> MAQQDGPTPEPSVGSRTVLVYMIAQNSLAPLASADIEEMKEGMRQVDATSGNLLVYIDDYSAPRLIRLGKDKKGKVVEETIENYPEQNSADANVMKKVISTAFNQYKAEKYGMVFWSHGEGWIPSPAKTR;> WFGQDGNNYMDIADLHAALQVAPDLDFLFFDACFMEAVEVAYALRDCGSYLISSPTEIPGPGAPYQTVVPAMFSAENAALKIASCYYDYYQSRYDDGIGMSNEDWTGGVSVGVAKMSELENLAVATSKVLPRYITGKQNFDLSGVMCYDRRTDK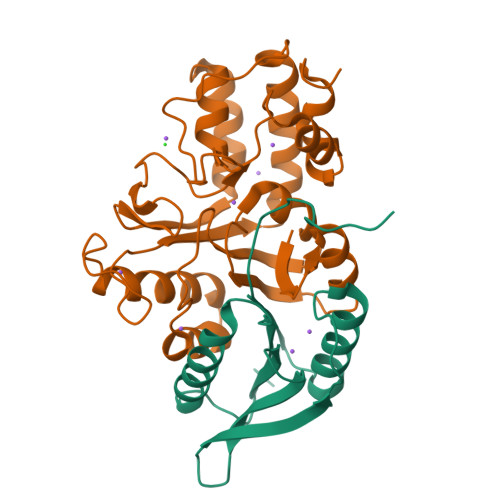QYYYDLDRFIYQITAGNGDYDSWREAFDKVMVYWKSTPRNYSAYAGMFTMNQDAKGLSTYIPRMSAPSLNTSYQQTEWYKVSGWADTGWYKNHHHHHH> PLREPRGLGPLQIWQTDFTLEPRMAPRSWLAVTVDTASSAIVVTQHGRVTSVAAQHHWATAIAVLGRPKAIKTDNGSCFTSKSTREWLARWGIAHTTGIPGNSQGQAMVERANRLLKDKIRVLAEGDGFMK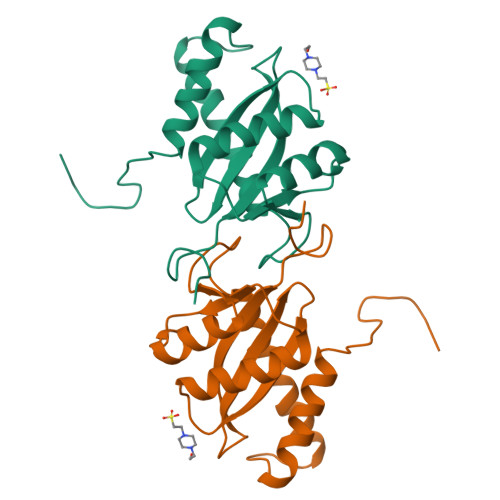RIPTSKQGELLAKAMYALNHFERGENTKTNL>ASMTGGQQMGRDEAGITGTWYNQLGSTFIVTAGADGALTGTYESAVGNAESRYVLTGRYDSAPATDGSGTALGWTVAWKNNYRNAHSATTWSGQYV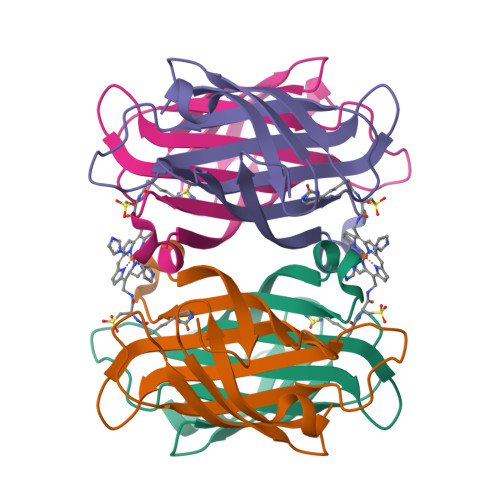GGAEARINTQWLLTAGTTEANAWASTLVGHDTFTKVKPSAASIDAAKKAGVNNGNPLDAVQQ[4x]> MSLSSPNILLTRIDNRLVHGQVGVTWTSTIGANLLVVV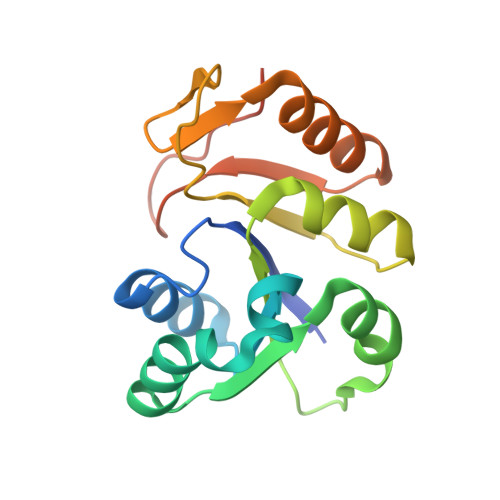DDVVANDDIQQKLMGITAETYGFGIRFFTIEKTINVIGKAAPHQKIFLICRTPQTVRKLVEGGIDLKDVNVGNMHFSEGKKQISSKVYVDDQDLTDLRFIKQRGVNVFIQDVPGDQKEQIPDEGHHHHHH> MGDAPSPEEKLHLITRNLQEVLGEEKLKEILKERELKIYWGTATTGKPHVAYFVPMSKIADFLKAGCEVTILFADLHAYLDNMKAPWELLELRVSYYENVIKAMLESIGVPLEKLKFIKGTDYQLSKEYTLDVYRLSSVVTQHDSKKAGAEVVKQVEHPLLSGLLYPGLQALDEEYLKVDAQFGGIDQRKIFTFAEKYLPALGYSKRVHLMNPMVPGLTGSKMSSSEEESKIDLLDRKEDVKKKLKKAFCEPGNVENNGVLSFIKHVLFPLKSEFVILRDEKWGGNKTYTAYVDLEKDFAAEVVHPGDLKNSVEVALNKLLDPIREKFNTPALKKLASAAYPDPSKQKPMAKGPAKNSEPEEV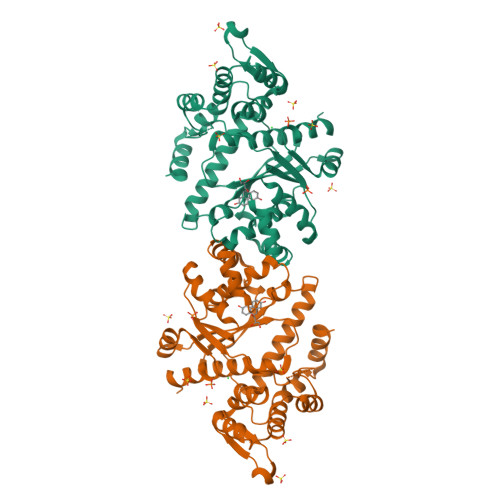ILEHHHHHH> MIYLSRLLIDTGGNPDRPRPGRKWLDNIYNVHRRLSMAFPSGLRREQDPHFLKPFSPNDFQKTPFLFRVDNNIDGNDKRAIIIVQSVLEPDWDYCFQNALDFLAAPPETKEYNPEFKAGQLLRFRLRVNASVRRHIPEMVQQDGQTIETGKILHKRVSLTWDASSTPDQALADWLAAKSPKLGF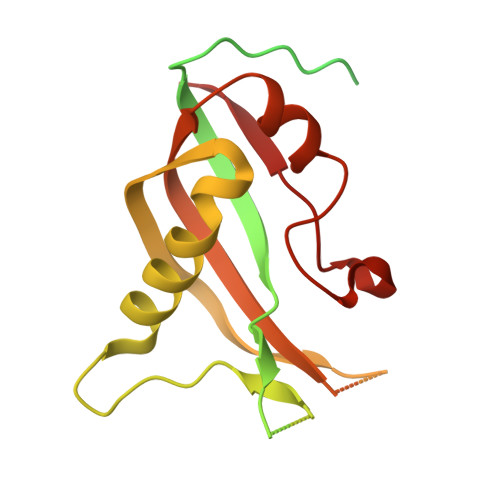TLQRCELLQLGWVYGSKPEPKNVKVKEQGQGYWREHKYNPLRFRAALLEGVLEVDDPKLFLKTLSSGIGKAKSFGFGLLSVLPIRNDG>GGRMKFTVEREHLLKPLQQVSGPLGGRPTLPILGNLLLQVADGTLSLTGTDLEMEMVARVALVQPHEPGATTVPARKFFDICRGLPEGAEIAVQLEGERMLVRSGRSRFSLSTLPAADFPNLDDWQSEVEFTLPQATMKRLIEATQFSMAHQDVRYYLNGMLFETEGEELRTVATDGHRLAVCSMPIGQSLPSHSVIVPRKGVIELMRMLDGGDNPLRVQIGSNNIRAHVGDFIFTSKLVDGRFP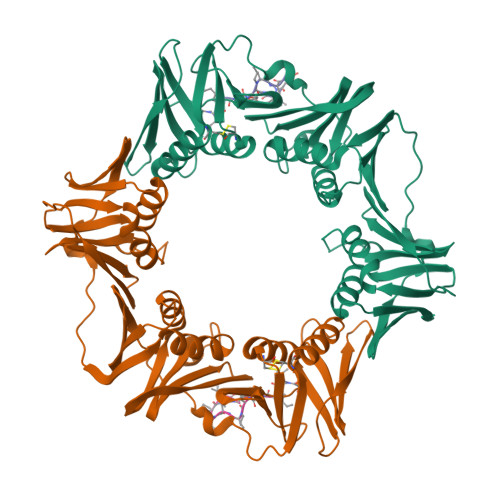DYRRVLPKNPDKHLEAGCDLLKQAFARAAILSNEKFRGVRLYVSENQLKITANNPEQEEAEEILDVTYSGAEMEIGFNVSYVLDVLNALKCENVRMMLTDSVSSVQIEDAASQSAAYVVMPMRL[2x]> SQQVDKIKASYPLFLDQDYKDMLAKKRDGFEEKYPQDKIDEVFQWTTTKEYQELNFQREALTVNPAKACQPLGAVLCALGFEKTMPYVHGSQGCVAHFRSYFNRHFREPVSC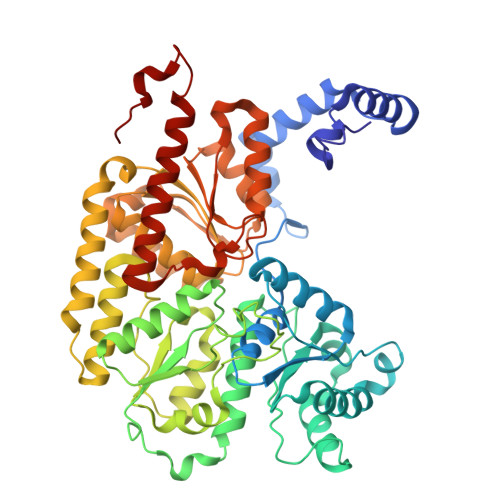VSDSMTEDAAVFGGQQNMKDGLQNCKATYKPDMIAVSTTCMAEVIGDDLNAFINNSKKEGFIPDEFPVPFAHTPSFVGSHVTGWDNMFEGIARYFTLKSMDDKVVGSNKKINIVPGFETYLGNFRVIKRMLSEMGVGYSLLSDPEEVLDTPADGQFRMYAGGTTQEEMKDAPNALNTVLLQPWHLEKTKKFVEGTWKHEVPKLNIPMGLDWTDEFLMKVSEISGQPIPASLTKERGRLVDMMTDSHTWLHGKRFALWGDPDFVMGLVKFLLELGCEPVHILCHNGNKRWKKAVDAILAASPYGKNATVYIGKDLWHLRSLVFTDKPDFMIGNSYGKFIQRDTLHKGKEFEVPLIRIGFPIFDRHHLHRSTTLGYEGAMQILTTLVNSILERLDEETRGMQATDYNHDLVR> EDAGLVAEAEAVAAGWMLDFLCLSLCRAFRDGRSEDFRRTRNSAEAIIHGLSSLTACQLRTIYICQFLTRIAAGKTLDAQFENDERITPLESALMIWGSIEKEHDKLHEEIQNLIKIQAIAVCMENGNFKEAEEVFERIFGDPNSHMPFKSKLLMII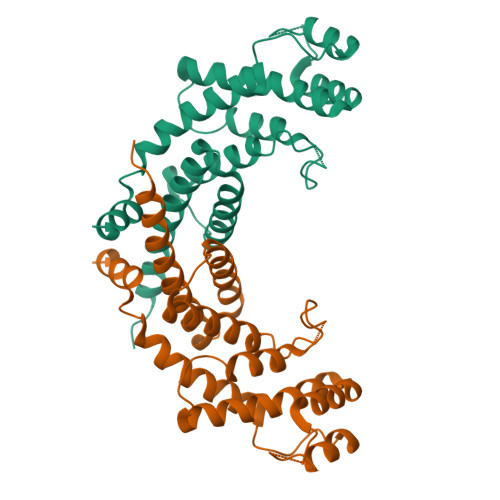SQKDTFHSFFQHFSYNHMMEKIKSYVNYVLSEKSSTFLMKAAAKVVE>AEAGITGTWYNQLGSTFIVTAGADGALTGTYESAVGNAESRYVLTGRYDSAPATDGSGTALGWTVAWKNNYRNAHSATTWSGQYVGGAEARINTQWLLTSGTTEANAWKSTLVGHDTFTKVKP[2x];>[2x]FCHP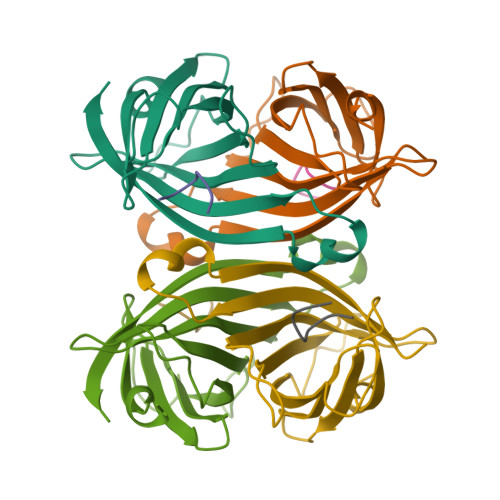QNTX5-CHLORO-2-({3-ISOBUTYL-4-[(5-PYRIDIN-4-YLPYRIMIDIN-2-YL)CARBONYL]PIPERAZIN-1-YL}SULFONYL)-1H-INDOLE 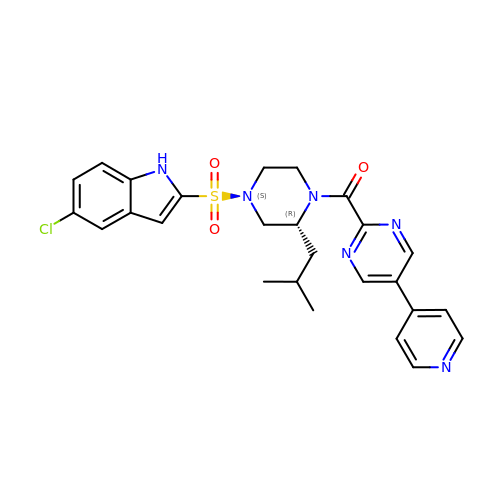| C26 H27 Cl N6 O3 S | JUUFKVAFKAKWRV-JOCHJYFZSA-N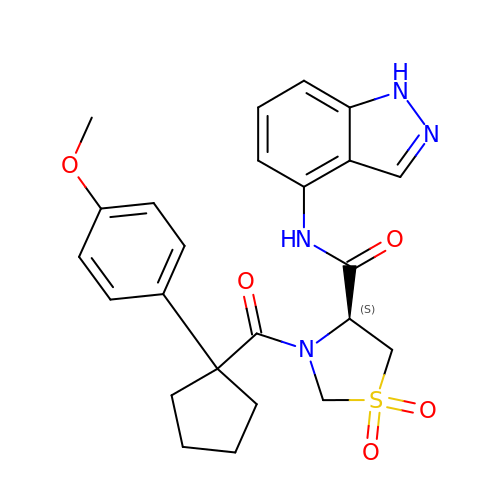(4S)-N-(3H-indazol-4-yl)-3-[1-(4-methoxyphenyl)cyclopentyl]carbonyl-1,1-bis(oxidanylidene)-1,3-thiazolidine-4-carboxamide | C24 H26 N4 O5 S | VWZAAFMUYDNGED-OAQYLSRUSA-N>[4x]MEVARGLEGVLFTESRMCYIDGQQGKLYYYGIPIQELAEKSSFEETTFLLLHGRLPRRQELEEFSAALARRRALPAHLLESFKRYPVSAH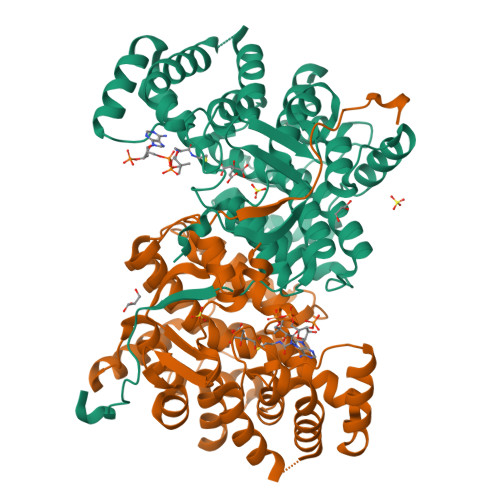PMSFLRTAVSEFGMLDPTEGDISREALYEKGLDLIAKFATIVAANKRLKEGKEPIPPREDLSHAANFLYMANGVEPSPEQARLMDAALILHAEHGFNASTFTAIAAFSTETDLYSAITAAVASLKGPRHGGANEAVMRMIQEIGTPERAREWVREKLAKKERIMGMGHRVYKAFDPRAGVLEKLARLVAEKHGHSKEYQILKIVEEEAGKVLNPRGIYPNVDFYSGVVYSDLGFSLEFFTPIFAVARISGWVGHILEYQELDNRLLRPGAKYVGELDVPYVPLEARE> 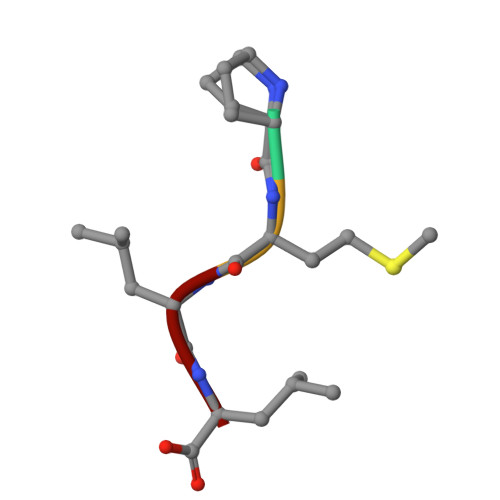PMLL>PFERGRTLAEQGDAARGIVACAGCHRADGGGDEALGAARLAGLEPAYLATQIERFRAGQRSHPVMSPWAERLTPVDIAAVSAYYGALAPASNARAPSDVDAAAGRALAETGDWPERDLPACVRCHGPGGVGAGAVFPPLAGQPYSYLLAQLQAWGTGRRHGEPMALMGAVAGRLDADEQRALAAYFATRPLAVADPADDLPDPSPPPATASVSTPAMTVAGANAVVPEHLGAVPAGRAEAASRFTPPSRDALPEGPLGEMVRLGARLFRHTNTDPRSAPHVGNDQTCAGCHLDNGRRADASPMWAAWVAYPAYRGKNQRVDTMAERIQGCFRYSMNAQDSVSGQVPETNGLVLDALQSYIFW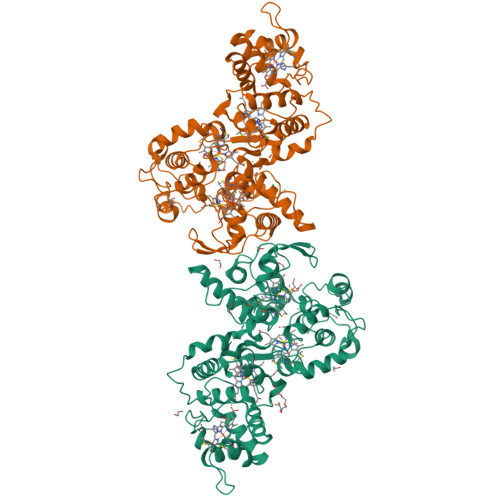LATGAPTGDTAMSGRGYPRLQPPAEGFDRTRGAALYAEHCALCHGAEGEGLLVDGEVVFPPLWGPRSYNWGAGMHRVDTAAAFIAANMPLLDTVRLTPQEAWDVAAYINAHERPQDPRFDGSVERTAARFHASPFDLYGEPLGVDGAVLGQGVAKDLEHHHHHH[2x]2-(4-methoxyphenyl)-N-{5-[2-oxo-2-(3-oxopiperazin-1-yl)ethoxy]pyridin-3-yl}acetamide 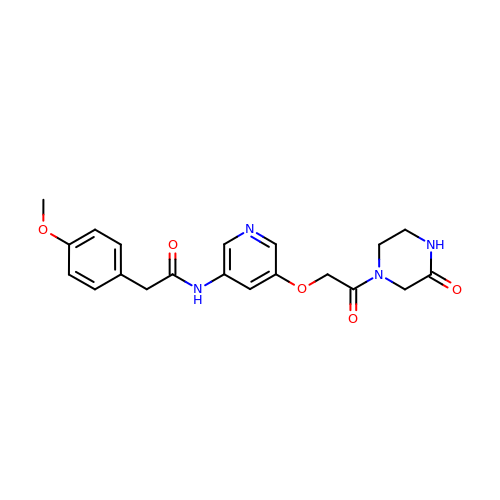| C20 H22 N4 O5 | HQORDXPKFUZBKB-UHFFFAOYSA-N> SMVRKNVNSLTPSEIENLRNALAAVQADKTDAGYQKIASFHGMPLSCQYPDGTAFACCQHGMVTFPHWHRLY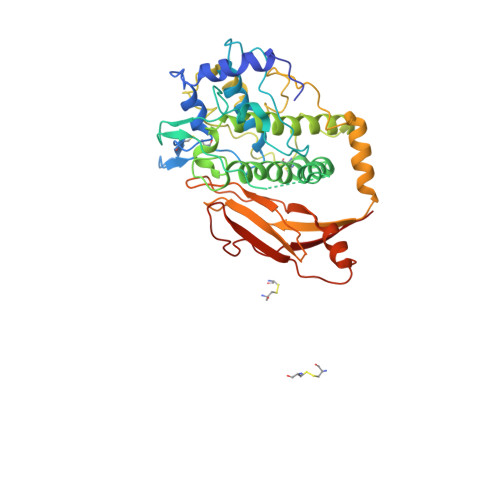MKQMEDALKAKGAKIGIPYWDWTTAFHSLPILVTEPKNNPFHHGYIDVADTKTTRDPRPQLFDDPEQGDQSFFYRQIAFALEQRDFCDFEIQFEMGHNAIHSWVGGPSPYGMSTLHYTSYDPLFYVHHSNTDRIWAIWQALQKYRGLPYNSANCEINKLKKPMMPFSSEDNPNEVTKAHSTGYKSFDYQQLNYEYDNLNFHGMTIPQLEVHLKKIQEKDRVFAGFLLRAIGQSADVNFDVCRKDGECTFGGTFCVLGGDYEMPWAFDRLFLYDISKSLVHLRLDAHDDFDIKVTIMGIDGKSLPPNLLPSPTILFKPGTGKI> MKPPQFTWAQWFETQHINMTSQQCTNAMQVINNYQRRCKNQNTFLLTTFANVVNVCGNPNMTCPSNKTRKNCHHSGSQVPLIHCNLTTPSPQNISNCRYAQTPANMFYI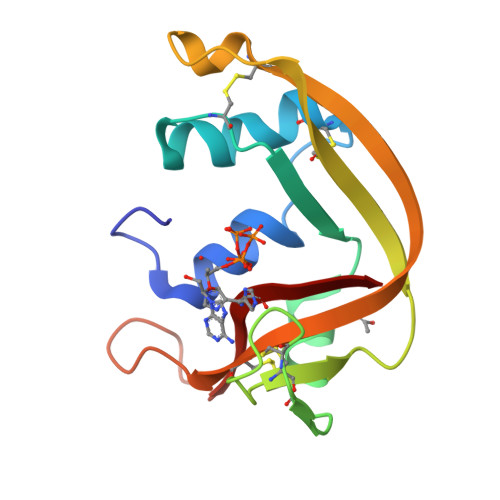VACDNRDQRRDPPQYPVVPVHLDRII> DIVSEKKPATEVDPTHFEKRFLKRIRDLGEGHFGKVELCRYDPEGDNTGEQVAVKSLKPESGGNHIADLKKEIEILRNLYHENIVKYKGICTEDGGNGIKLIMEFLPSGSLKEYLPKNKNKINLKQQLKYAVQICKGMDYLGSRQYVHRDLAARNVLVESEHQVKIGDFGLTKAIETDKEYYTVKDDRDSPVFWYAPECLMQSKFYIASDVWSFGVTLHELLTYCDSDSSPMALFLKMIGPTHGQMTVTRLVNTLKEGKRLPCPPNCPDEVYQLMRKCWEFQPSNRTSFQNLIEGF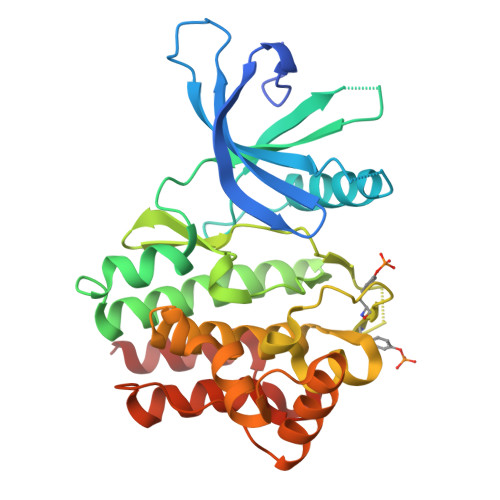EALLK> PDPKGGNLTPFIHKEGERSLQGILDNLGGRGKKTPGTAAGLFIASPNTENPNYYYTWTRDSALTAKCLIDLFEDSRAVFPIDRKYLETGIRDYVSSQAILQSVSNPSGTLKDGSGLGEPKFEIDLNPFSGAWGRPQRDGPALRATAMITYANYLISHGQKSDVSQVMWPIIANDLAYVGQYWNNTGFDLWEEVDGSSFFTIAVQHRALVEGSQLAKKLGKSCDACDSQPPQILCFLQSFWNGKY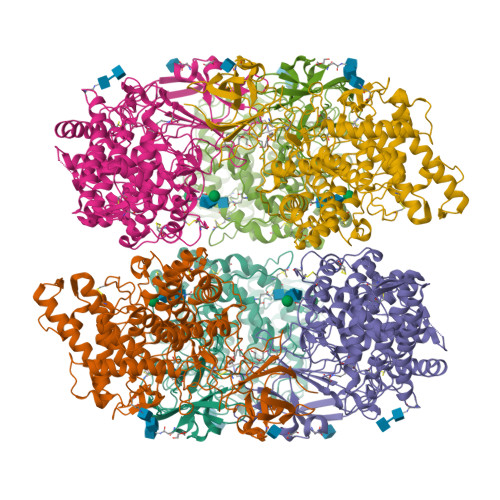ITSNINTQASRSGIDLDSVLGSIHTFDPEAACDDATFQPCSARALANHKVYVDSFRSIYKINAGLAEGSAANVGRYPEDVYQGGNPWYLATLGASELLYDALYQWDRLGKLEVSETSLSFFKDFDATVKIGSYSRNSKTYKKLTQSIKSYADGFIQLVQQYTPSNGSLAEQYDRNTAAPLSANDLTWSFASFLTATQRRDAVVPPSWGAKSANKVPTTCSASPVVGTYKAPTATFSSKTKCVPAKDIVPITFYLIENTYYGENVFMSGNITALGNWDAKKGFPLTANLYTQDQNLWFASVEFIPAGTPFEYKYYKVEPNGDITWEKGPNRVFVAPTGCPVQPHSNDVWQF>[4x]MKKRIINAPTLETLAMLKRRMPSESRNRLEMVRIDAI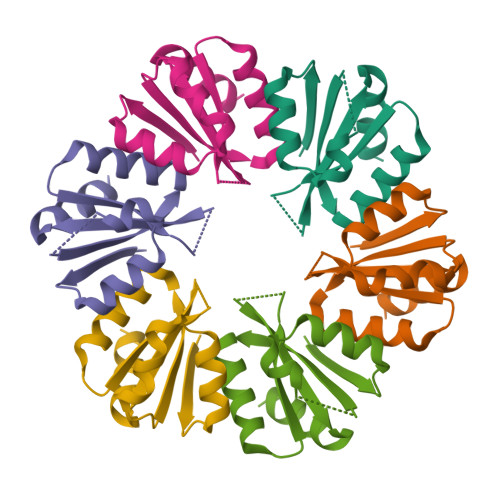GLIMLPVPDLYFYADQASKSAHVAVSEIFGSCPQHITTLAIFGEVAAVNEAMRIIEDDASTFLEHHHHHH> MASAATGVRAVPGNENSLEIEELARFAVDEHNKKENALLEFVRVVKAKEQIDLTQEWVFTMYYLTLEAKDGGKKKLYEAKVWVKGLTNWKLGMNFKELQEFKPVGDAAAAHHHHHH;> MNNDHINLKVAGQDGSVVQFKIKRHTPLSKLMKAYCERQGLSMRQIRFRFDGQP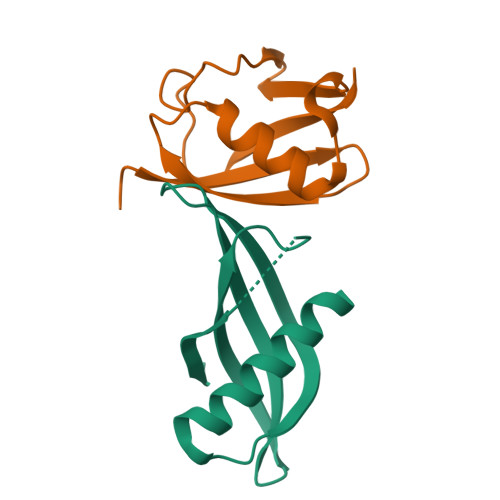INETDTPAQLEMEDEDTIDVFQQ>MGLNYNQEDFMGLDRFFQDAVSHNNTDANAASSIEVEMYECDCMYPTFAEIARRSGQPEIGAMFDAIAKEEGMHAQLLTKLYSELEVKDSAETLEAKRLVSTIESQIDAVASDSRGLRRALETALEVETIESQKTYPAFAKLAAEQ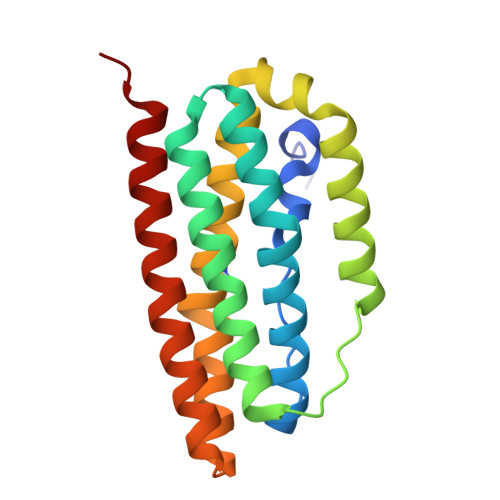GNMEVATAFEAIVKSETKHANWVKRALENLLEVA[2x]Here, we report the complete structure of a bimodular ∼760 kDa BoNT/A large progenitor toxin complex (L-PTC), which is composed of BoNT and four non-toxic bacterial proteins. We found that L-PTC/A consists of two structurally and functionally independent sub-complexes, the M-PTC and the HA complex. The HA complex is composed of HA70, HA17, and HA33 in a 3∶3∶6 stoichiometry and adopts an extended three-blade architecture, whereas the M-PTC is situated on top of the HA complex platform. BoNT/A absorption is mainly mediated by nine glycan-binding sites on the HA complex that together form multivalent interactions with host carbohydrate receptors on intestinal epithelial cells.

We next separated the HA complex into two major components: the central hub composed of homo-trimeric HA70 and the blade composed of HA70D3–HA17–HA33. Their crystal structures were determined at 2.9 Å and 3.7 Å, respectively. HA70 consists of three domains (D1–3). The D1 and D2 domains, which adopt similar structures, mediate the trimerization of HA70 with each protomer contributing ∼3,100 Å2 of solvent-accessible area for interactions. The D3 domain, sitting at the tip of the trimer, is composed of two similar jelly-roll-like β-sandwich structures. The linker between D1 and D2 (residues Thr190–Ser205) is degraded and not visible in the crystal structure, which is reminiscent of the post-translational nicking of HA70 into ∼25 and ∼45 kDa fragments that occurs physiologically. Gly399 and Ile400 of HA70 are located in a loop that has weak electron density in the crystal structures, suggesting high flexibility. The corresponding interface residues in the HA complex are located around the center of the HA70 trimer.

> GSNSSIKKIYNDIQEKVINYSDTIDLADGNYVVRRGDGWILSRQNQILGGSVISNGSTGIVGDLRVNDNAIPYYYPTPSFNEEYIKNNIQTVFTNFTEANQIPIGFEFSKTAPSNKNLYMYLQYTYIRYEIIKVLQHEIIERAVLYVPSLGYVKSIEFNPGEKINKDFYFLTNDKCILNEQFLYKKILET;> TQRVLPYSNGLYVINKGDGYIRTNDKDLIGTLLIEAGSSGSIIQPRLRNTTRPLFTTSNDTKFSQQYTEERLKDAFNVQLFNTSTSLFKFVEEAPSDKNICIKAYNTYEKYELIDYQNGSIVNKAEYYLPSLGYCEVTNAPSPESEVVKMQVAEDGFIQNGPEEEIVVGVIDPSENIQEINTAISDNYTYNIPGIVNNNPFYILFTVNTTGIYKINAQNNLPSLKIYEAIGSGNRNFQSGNLCDDDIKAINYITGFDSPNAKSYLVVLLNKDKNYYIRVPQTSSNIENQIQFKREEGDLRNLMNSSVNIIDNLNSTGAHYYTRQSPDVHDYISYEFTIPGNFNNKDTSNIRLYTSYNQGIGTLFRVTETIDGYNLINIQQNLHLLNNTNSIRLLNGAIYILKVEVTELNNYNIRLHIDITNPGSAWSHPQFEK> GPMLQKREKVLLLRTFQGRTLRIVREHYLRPCVPCHSPLCPQPAACSHDGKLLSSDVTHYVIPDWK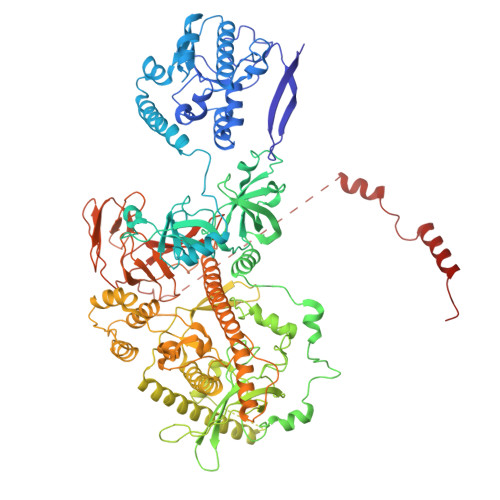VVQDYLEILEFPELKGIIFMQTACQAVQHQRGRRQYNKLRNLLKDARHDCILFANEFQQCCYLPRERGESMEKWQTRSIYNAAVWYYHHCQDRMPIVMVTEDEEAIQQYGSETEGVFVITFKNYLDNFWPDLKAAHELCDSILQSRRERENESQESHGKEYPEHLPLEVLEAGIKSGRYIQGILNVNKHRAQIEAFVRLQGASSKDSDLVSDILIHGMKARNRSIHGDVVVVELLPKNEWKGRTVALCENDCDDKASGESPSEPMPTGRVVGILQKNWRDYVVTFPSKEEVQSQGKNAQKILVTPWDYRIPKIRISTQQAETLQDFRVVVRIDSWESTSVYPNGHFVRVLGRIGDLEGEIATILVENSISVIPFSEAQMCEMPVNTPESPWKVSPEEEQKRKDLRKSHLVFSIDPKGCEDVNDTLSVRTLNNGNLELGVHIADVTHFVAPNSYIDIEARTRATTYYLADRRYDMLPSVLSADLCSLLGGVDRYAVSIMWELDKASYEIKKVWYGRTIIRSAYKLFYEAAQELLDGNLSVVDDIPEFKDLDEKSRQAKLEELVWAIGKLTDIARHVRAKRDGCGALELEGVEVCVQLDDKKNIHDLIPKQPLEVHETVAECMILANHWVAKKIWESFPHQALLRQHPPPHQEFFSELRECAKAKGFFIDTRSNKTLADSLDNANDPHDPIVNRLLRSMATQAMSNALYFSTGSCAEEEFHHYGLALDKYTHFTSPIRRYSDIVVHRLLMAAISKDKKMEIKGNLFSNKDLEELCRHINNRNQAAQHSQKQSTELFQCMYFKDKDPATEERCISDGVIYSIRTNGVLLFIPRFGIKGAAYLKNKDGLVISCGPDSCSEWKPGSLQRFQNKITSTTTDGESVTFHLFDHVTVRISIQASRCHSDTIRLEIISNKPYKIPNTELIHQSSPLLKSELVKEVTKSVEEAQLAQEVKVNIIQEEYQEYRQTKGRSLYTLLEEIRDLALLDVSNNYGI>[6x]RSRIFKIIVIGDSNVGKTCLTYRFCAGRFPDRTEATIGVDFRERAVDIDGERIKI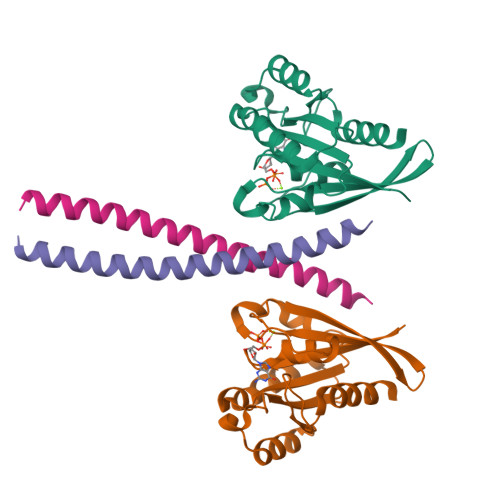QLWDTAGLERFRKSMVQHYYRNVHAVVFVYDMTNMASFHSLPAWIEECKQHLLANDIPRILVGNKCDLRSAIQVPTDLAQKFADTHSMPLFETSAKNPNDNDHVEAIFMTLAHKLKSH;>DLEVANQTLKDEYDALQITFTALEEKLRKTTEENQELVTRWMAEKAQEANRLNAENE[6x]> SNAMRPFQVQIPQADIDDLKRRLSETRWPELVDVGWSRGAPLSYIKELAEYWRDGFDWRAAERRINQYPQFTTEIDGATIHFLHVRSPEPDATPMVITHGWPGTPVEFLDIIGPLTDPRAHGGDPADAFHLVIPSLPGFGLSGPLKSAGWELGRIAMAWSKLMASLGY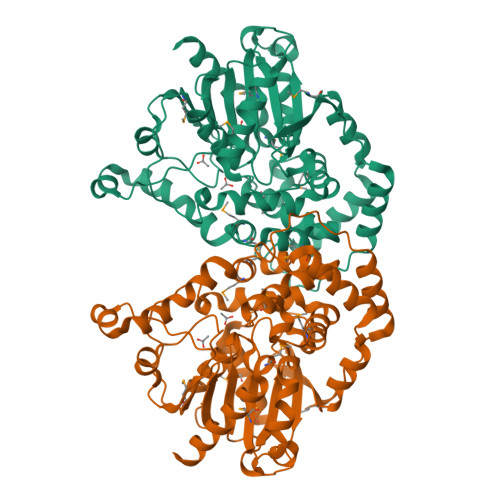ERYIAQGGDIGAFTSLLLGAIDPSHLAGIHVNLLQTNLSGEPGELETLSDADKARLAVSERFLDDLSGPMKMQSTRPHTIGYMLNDSPVAQLAYLLEMFKHWAQTENVPEDAVDRDLMLTHISLFWFTATGGSAAQAHYELKPFLPITSLIGRSPTLDVPMGVAVYPGALFQPVRSLAERDFKQIVHWAELDRGGHFSAMEEPDLFVDDLRTFNRTLKKL>[4x]MGSDKIHHHHHHMKIDILDKGFVELVDVMGNDLSAVRAARVSFDMGLKDEERDRHLIEYLMKHGHETPFE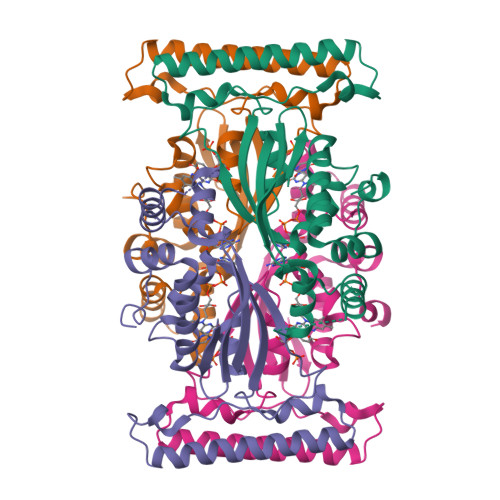HIVFTFHVKAPIFVARQWFRHRIASYNELSGRYSKLSYEFYIPSPERLEGYKTTIPPERVTEKISEIVDKAYRTYLELIESGVPREVARIVLPLNLYTRFFWTVNARSLMNFLNLAADSHAQWEIQQYALAIARIFKEKCPWTFEAFLKYAYKGDILKEVQV>MSGADRSPNAGAAPDSAPGQAAVASAYQRFEPRAYLRNNYAPPRGDLCNPNGVGPWKLRCLAQTFATGEVSGRTLIDIGSGPTVYQLLSACSHFEDITMTDFLEVNRQELGRWLQEEPGAFNWSMYSQHACLIEGKGECWQDKERQLRARVKRVLPIDVHQPQPLGAGSPAPLPADALVSAFCLDAVSPDLASFQRALDHITTLLRPGGHLLLIGALEESWYLAGEARLTV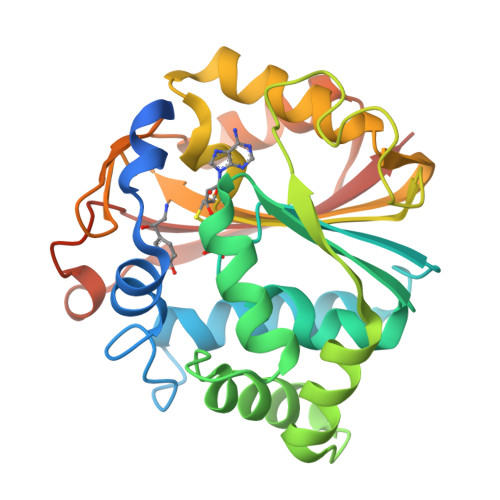VPVSEEEVREALVRSGYKVRDLRTYIMPAHLQTGVDDVKGVFFAWAQKVGLEHHHHHH[2x]> GPVWRKHYITYRINNYTPDMNREDVDYAIRKAFQVWSNVTPLKFSKINTGMADILVVFARGAHGDDHAFDGKGGILAHAFGPGSGIGGDAHFDEDEFWTTHSGGTNLFLTAVH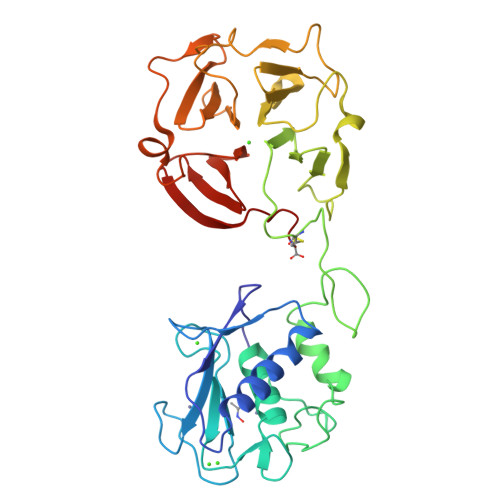EIGHSLGLGHSSDPKAVMFPTYKYVDINTFRLSADDIRGIQSLYGDPKENQRLPNPDNSEPALCDPNLSFDAVTTVGNKIFFFKDRFFWLKVSERPKTSVNLISSLWPTLPSGIEAAYEIEARNQVFLFKDDKYWLISNLRPEPNYPKSIHSFGFPNFVKKIDAAVFNPRFYRTYFFVDNQYWRYDERRQMMDPGYPKLITKNFQGIGPKIDAVFYSKNKYYYFFQGSNQFEYDFLLQRITKTLKSNSWFGC>MAGARRLELGEALALGSGWRHACHALLYAPDPGMLFGRIPLRYAILMQMRFDGRLGFPGGFVDTQDRSLEDGLNRELREELGEAAAAFRVERTDYRSSHVGSGPRVVAHFYAKRLTLEELLAVEAGATRAKDHGL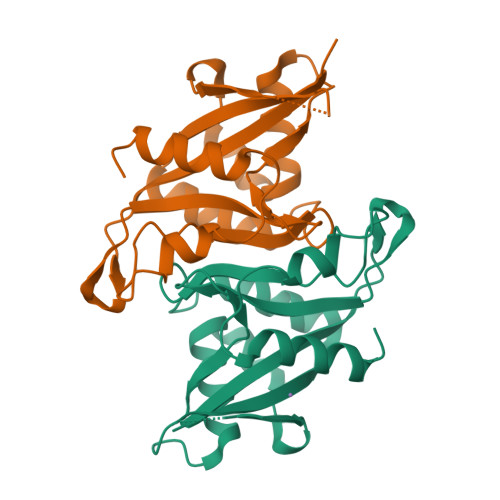EVLGLVRVPLYTLRDGVGGLPTFLENSFIGSAREQLLEALQDLGLLQSGSISGLKIPAHH[4x]> AMADIGSEGHRTLASTPALWASIPCPRSELRLDLVLPSGQSFRWREQSPAHWSGVLADQVWTLTQTEEQLHCTVYRGDKSQASRPTPDELE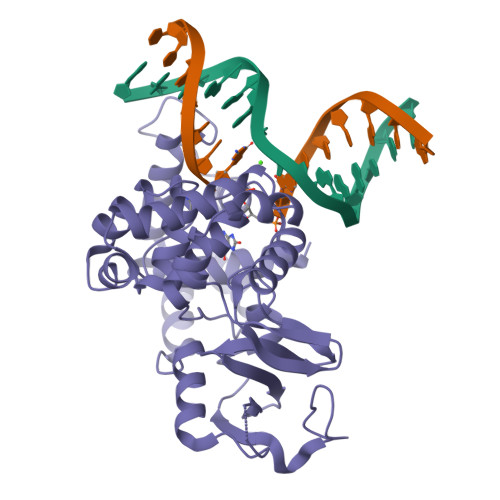AVRKYFQLDVTLAQLYHHWGSVDSHFQEVAQKFQGVRLLRQDPIECLFSFICSSNNNIARITGMVERLCQAFGPRLIQLDDVTYHGFPSLQALAGPEVEAHLRKLGLGYRARYVSASARAILEEQGGLAWLQQLRESSYEEAHKALCILPGVGTKVADCICLMALDKPQAVPVDVHMWHIAQRDYSWHPTTSQAKGPSPQTNKELGNFFRSLWGPYAGWAQAVLFSADLRQSR>MKTIFSGIQPSGVITIGNYIGALRQFVELQHEYNCYFCIVDQHAITVWQDPHELRQNIRRLAALYLAVGIDPTQATLFIQSEVPAHAQAAWMLQCIVYIGELERMTQFKEKSAGKEAVSAGLLTYPPLMAADILLYNTDIVPVGEDQKQHIELTRDLAERFNKRYG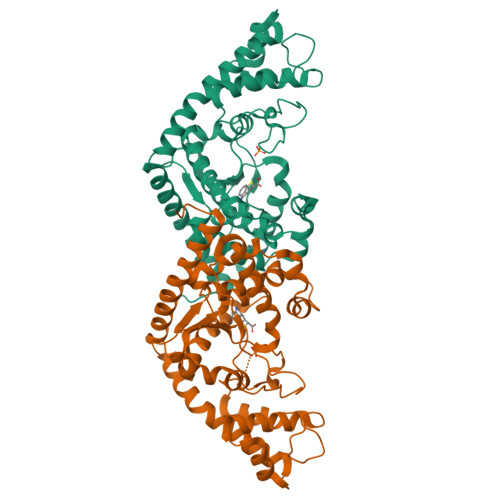ELFTIPEARIPKVGARIMSLVDPTKKMSKSDPNPKAYITLLDDAKTIEKKIKSAVTDSEGTIRYDKEAKPGISNLLNIYSTLSGQSIEELERQYEGKGYGVFKADLAQVVIETLRPIQERYHHWMESEELDRVLDEGAEKANRVASEMVRKMEQAMGLGRRR[2x]> MSEYRPSRPSNPR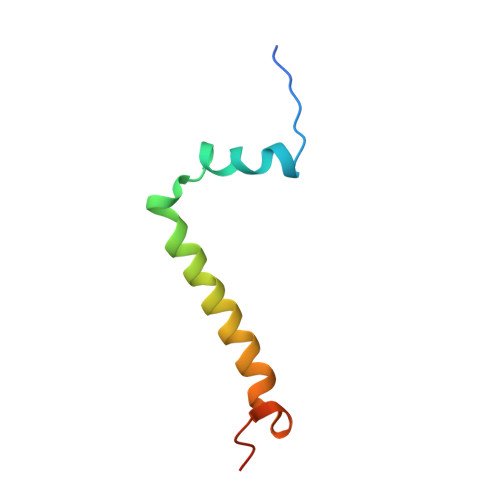DDWKLWLVVNPGTWLIPLLITFLATALIVHSFVFTHEAYNPLTYEVSE> ASDYCKVIFPYEAQNDDELTIKEGDIVTLINKDCIDVGWWEGELNGRRGVFPDNFVKLLPPLEHHHHHH

Several lines of evidence support a role of CMS/CIN85 (Cas ligand with Multiple SH3 domains/Cbl-Interacting protein of 85 kDa) in the regulation of Cbl-directed RTK down regulation. CMS, also known as CD2AP (CD2 associated protein), shares overall domain organization with CIN85, containing three SH3 (Src-Homology) domains, a proline-rich region and a coiled-coiled domain, and high sequence identity and hence, it has been assumed to belong to the same family of ubiquitously expressed adaptor molecules and elicit similar biological functions. Recently, SH3 domains were identified as a new class of UBDs. In the current work, we have performed structural and mutational analysis of the three SH3 domains of CD2AP and the third SH3 domain of CIN85.

In light of these results, and due to the higher CIN85 SH3-C affinity to C-terminal GST-tagged ubiquitin reported before, a NMR detected titration was carried out with unlabelled CIN85 SH3-C and 15N-labelled C-terminal His-tagged ubiquitin. Interestingly, our NMR titrations suggest significantly tighter binding as well as different areas affected in ubiquitin upon binding compared to those previously reported by Forman-Kay and co-workers using non-tagged ubiquitin. Furthermore, the ubiquitin areas targeted in this work are very similar to the CD2AP SH3-C titration. According to these results and the high sequence identity (53.3%) between the two SH3-C domains, we produced the CIN85 F322Y SH3-C mutant and titrated increasing amounts of it into 15N labelled ubiquitin. Although it was stated that this mutant abolishes ubiquitin binding due to the replacement of the key Phe322 residue as in Sla1 SH3-3, we observed binding with a similar affinity to that observed for the wild type form, indicating that CIN85 SH3-C displays a comparable behaviour to CD2AP SH3-C towards ubiquitin binding. Bigger differences are observed within the n-Src loop. This loop in CD2AP and CIN85 SH3-C is one residue longer, resulting in a different position of the sidechains and creating a shallow and highly negatively charged groove with the RT loop, accommodating the ubiquitin C-terminus on its surface. Furthermore, the F322Y mutation in the CIN85 SH3-C domain does not diminish ubiquitin binding, and taking also into account the higher affinity of CIN85 SH3-C towards C-terminal tagged ubiquitin molecules, we can conclude that CIN85 and CD2AP SH3-C domains present a similar ubiquitin binding mode. These results are in contrast to the relative orientation of the CIN85 SH3-C domain and ubiquitin in the previously determined complex; the difference might be the result of a distortion due to the G76C mutation and the incorporation of a MTSL molecule into the ubiquitin C-terminus, as well as due to PRE constraints sensitive to minor alternate conformations.The mGeos series of rsFP’s display similar switching behavior to Dronpa. The series was developed from mEos2, with mutations that remove the undesirable irreversible green-to-red photo conversation, increase fluorescence brightness and provide high thermal stability of the off-state. Skylan-NS represents a further improvement, with reduced per cycle bleaching and higher photoswitching quantum yield in the on→off than Dronpa. We present high resolution room temperature SFX structures of Skylan-NS in both ‘on’ and meta-stable ‘off’ state collected using two different XFELs, the SPring-8 Angstrom Compact free electron Laser (SACLA), Japan and the Linear Coherent Light Source (LCLS), USA.

We collected datasets for the dark on-state using two different methods at the SACLA/EH4 station using the DAPHNIS chamber. For comparison, we obtained complementary data using the droplet-on-demand method for the dark on-state, using smaller crystals than those used for the grease method, which were delivered in the crystallization mother liquor. The hit-rate could be carefully controlled with the crystal density, and levels of 40% could be sustained with crystal densities of 4.8 × 107–9 × 107 crystal/mL. Table 1 shows the CC* and R-split values that reveal data from the droplet method was lower quality than that obtained from the grease injection method. The comparison between the two on-state structures collected with the grease injection and droplet methods under the same conditions (Black) showed the lowest R-factor over the intermediate resolution range up to ≈3 Å resolution. An increase of the R-factor for the increased resolution (<3 Å) is likely indicative of genuine structural differences between the grease and droplet methods, in agreement with the observed degradation of R-split and CC* when merging intensities together (Black). The R-factor for the on- and off-state experiments using the droplet methods (green) (but at different photon energy) is considerably higher than the two off-state measurements conducted at different facilities, including the lower resolution reflections. Following complete refinement of all four datasets, both on-state structures showed no statistically significant density in either the 2Fobs-Fcalc or the Fobs-Fcalc maps that could be assigned to a trans chromophore structure. The same was observed for chromophore omit maps, that also, at lower sigma levels, did not show such density. This is in agreement with the dark incubation and dark sample injection which corresponds to a 100% on-state concentration. Photoisomerisation is clearly seen in a comparison of the “on” and “off” refined structures where the dihedral angle of the chain connecting the phenol ring to the rest of the chromophore (N–C=C–C) changes from 1° (cis) → 171.1° (trans) in the on- vs the off-state and the pheonolic oxygen is displaced by 6.2 Å.

> SAIKPDMKIKLRMEGNVNGHHFVIDGDGTGKPFEGKQSMDLEVKEGGPLPFAFDILTTAFLYGNRVFAKYPDNIQDYFKQSFPKGYSWERSLTFEDGGICNARNDITMEGDTFYNKVRFYGTNFPANGPVMQKKTLKWEPSTEKMYVRDGVLTGDVEMALLLEGNAHYRCDFRTTYKAKEKGVKLPGAHFVDHCIEILSHDKDYNKVKLYEHAVAHSGLPDNARR>MAGIKVFGHPASIATRRVLIALHEKNLDFELVHVELKDGEHKKEPFLSRNPFGQVPAFEDGDLKLFESRAITQYIAHRYENQGTNLLQTDSKNISQYAIMAIGMQVEDHQFDPVASKLAFEQIFKSIYGLT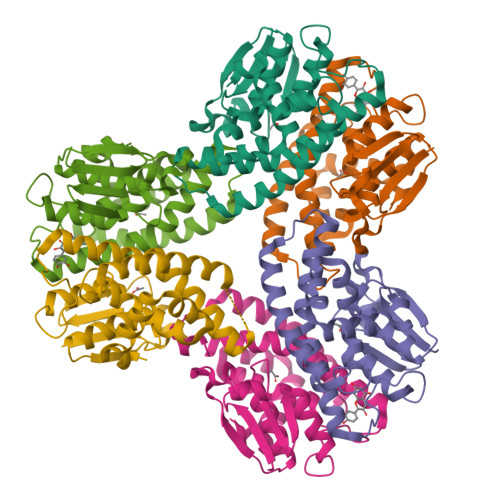TDEAVVAEEEAKLAKVLDVYEARLKEFKYLAGETFTLTDLHHIPAIQYLLGTPTKKLFTERPRVNEWVAEITKRPASEKVQ[6x]>MSFRVSASSSVKPEKDIRIGLLGA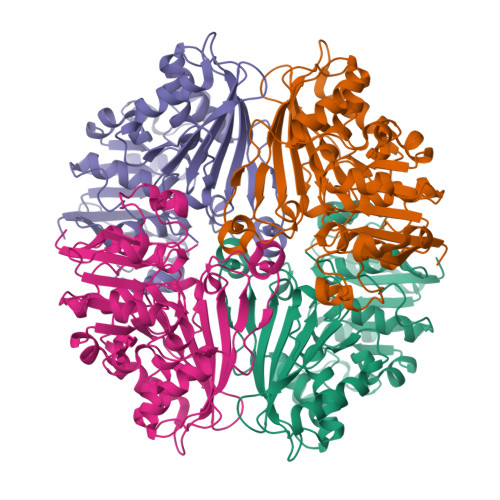SGYTGAEIVRLLANHPHFQVTLMTADRKAGQSMESVFPHLRAQKLPTLVSVKDADFSTVDAVFCCLPHGTTQEIIKELPTALKIVDLSADFRLRNIAEYEEWYGQPHKAVELQKEVVYGLTEILREDIKKARLVANPGCYPTTIQLPLVPLLKANLIKHENIIIDAKSGVSGAGRGAKEANLYSEIAEGISSYGVTRHRHVPEIEQGLSDVAQSKVTVSFTPHLMPMIRGMQSTIYVEMAPGVRTEDLHQQLKTSYEDEEFVKVLDEGVVPRTHNVRGSNYCHMSVFPDRIPGRAIIISVIDNLVKGASGQALQNLNIMLGYPETTGLLHQPLFP[4x]>AQSVPYGISQIKAPALHSQGYTGSNVKVAVIDSGIDSSHPDLNVRGGASFVPSETNPYQDGSSHGTHVAGTIA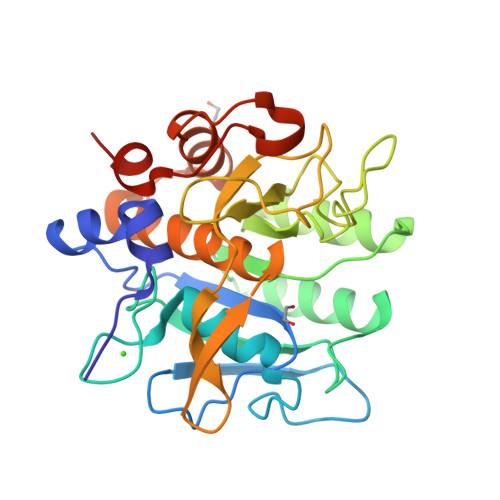ALNNSIGVLGVAPSASLYAVKVLDSTGSGQYSWIINGIEWAISNNMDVINMSLGGPSGSTALKTVVDKAVSSGIVVAAAAGNEGQHPKEGSTVGYPAKYPSTIAVGAVNSSNQRASFSSAGSELDVMAPGVSIQSTLPGGTYGAYNGTCMATPHVAGAAALILSKHPTWTNAQVRDRLESTATYLGNSFYYGKGLINVQAAAQSLEHHHHHH[2x]>[2x]MGSSHHHHHHSSLVPRGSHMMETKNENSDVSRAEEFKSQANEAFKGHKYSSAIDLYTKAIELNSNNAVYWA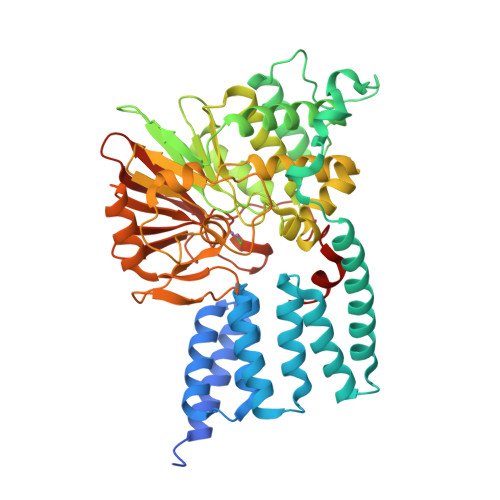NRAFAHTKLEEYGSAIQDASKAIEVDSRYSKGYYRRGAAYLAMGKFKDALKDFQQVKRLSPNDPDATRKLKECEKAVMKLKFEEAISVPVSERRSVAESIDFHTIEVEPQYSGARIEGEEVTLDFVKTMMEDFKNQKTLHKRYAYQIVLQTRQILLALPSLVDISVPHGKHITVCGDVHGQFYDLLNIFELNGLPSEENPYLFNGDFVDRGSFSVEIILTLFAFKCMCPSSIYLARGNHESKSMNKIYGFEGEVRSKLSEKFVDLFAEVFCYLPLAHVINGKVFVVHGGLFSVDGVKLSDIRAIDRFCEPPEEGLMCELLWSDPQPLPGRGPSKRGVGLSFGGDVTKRFLQDNNLDLLVRSHEVKDEGYEVEHDGKLITVFSAPNYCDQMGNKGAFIRFEAPDMKPNIVTFSAVPHPDVKPMAYANNFLRMFN> MHHHHHHMSKFTWKELIQLGSPSKAYESSLACIAHIDMNAFFAQVEQMRCGLSKEDPVVCVQWNSIIAVSYAARKYGISRMDTIQEALKKCSNLIPIHTAVFKKGEDFWQYHDGCGSWVQDPAKQISVEDHKVSLEPYRRESRKALKIFKSACDLVERASIDEVFLDLGRICFNMLMFDNEYELTGDLKLKDALSNIREAFIGGNYDINSHLPLIPEKIKSLKFEG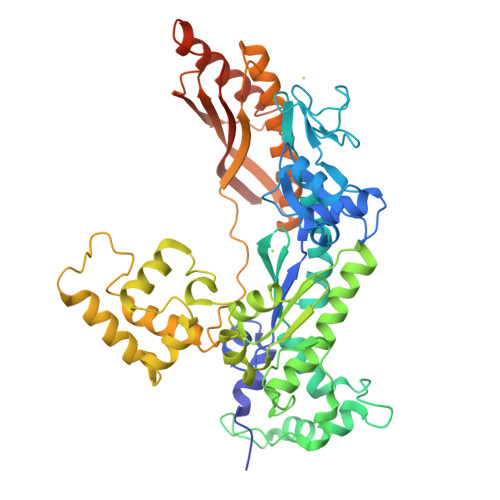DVFNPEGRDLITDWDDVILALGSQVCKGIRDSIKDILGYTTSCGLSSTKNVCKLASNYKKPDAQTIVKNDCLLDFLDCGKFEITSFWTLGGVLGKELIDVLDLPHENSIKHIRETWPDNAGQLKEFLDAKVKQSDYDRSTSNIDPLKTADLAEKLFKLSRGRYGLPLSSRPVVKSMMSNKNLRGKSCNSIVDCISWLEVFCAELTSRIQDLEQEYNKIVIPRTVSISLKTKSYEVYRKSGPVAYKGINFQSHELLKVGIKFVTDLDIKGKNKSYYPLTKLSMTITNFDIIDLQKTVVDMFGNQVHTFKS>[4x]GSHMYMEKLRLDNRVAIVTGGAQNIGLACVTALAEAGARVIIADLDEAMATKAVEDLRMEGHDVSSVVMDVTNTESVQNAVRSV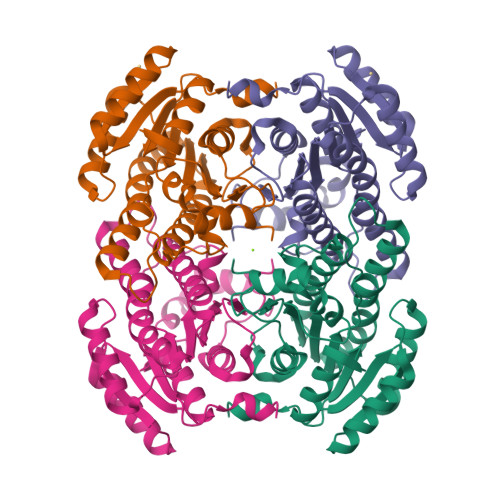HEQEGRVDILVACAGICISEVKAEDMTDGQWLKQVDINLNGMFRSCQAVGRIMLEQKQGVIVAIGSMSGLIVNRPQQQAAYNASKAGVHQYIRSLAAEWAPHGIRANAVAPTYIETTLTRFGMEKPELYDAWIAGTPMGRVGQPDEVASVVQFLASDAASLMTGAIVNVDAGFTVW>MAASGLDHLKNGYRRRFCRPSRARDINTEQGQNVLEILQDCFEEKSLANDFSTNSTKSVPNSTRKIKDTCIQSPSKECQKSHPKSVPVSSKKKEASLQFVVEPSEATNRSVQAHEVHQKILATDVSSKNTPDSKKISSRNINDHHSEADEEFYLSVGSPSVLLDAKTSVSQNVIPSSAQKRETYTFENSVNMLPSSTEVSVKTKKRLNFDDKVMLKKIEIDNKVSDEEDKTSEGQERKPSGSSQNRIRDSEYEIQRQAKKSFSTLFLETVKRKSESSPIVRHAATAPPHSCPPDDTKLIEDEFIIDESDQSFASRSWITIPRKAGSLKQRTISPAESTALLQGRKSREKHHNILPKTLANDKHSHKPHPVETSQPSDKTVLDTSYALIGETVNNYRSTKYEMYSKNAEKPSRSKRTIKQKQRRKFMAKPAEEQLDVGQSKDENIHTSHITQDEFQRNSDRNMEEHEEMGNDCVSKKQMPPVGSKKSSTRKDKEESKKKRFSSESKNKLVPEEVTSTVTKSRRISRRPSDWWVVKSEESPVYSNSSVRNELPMHHNSSRKSTKKTNQSSKNIRKKTIPLKRQKTATKGNQRVQKFLNAEGSGGIVGHDEISRCSLSEPLESDEADLAKKKNLDCSRSTRSSKNEDNIMTAQNVPLKPQTSGYTCNIPTESNLDSGEHKTSVLEESGPSRLNNNYLMSGKNDVDDEEVHGSSDDSKQSKVIPKNRIHHKLVLPSNTPNVRRTKRTRLKPLEYWRGERIDYQGRPSGGFVISGVLSPDTISSKRKAKENIGKVNKKSNKKRICLDNDERKTNLMVNLGIPLGDPLQPTRVKDPETREIILMDLVRPQDTYQFFVKHGELKVYKTLDTPFFSTGKLILGPQEEKGKQHVGQDILVFYVNFGDLLCTLHETPYILSTGDSFYVPSGNYYNIKNLRNEESVLLFTQIKR[2x];> MEEQPQMQDADEPADSGGEGRAGGPPQVAGAQAACSEDRMTLLLRLRAQTKQQLLEYKSMVDASEEKTPEQIMQEKQIEAKIEDLENEIEEVKVAFEIKKLALDRMRLSTALKKNLEKISRQSSVLMDNMKHLLELNKLIMKSQQESWDLEEKLLDIRKKRLQLKQASESKLLEIQTEKNKQKIDLDSMENSERIKIIRQNLQMEIKITTVIQHVFQNLILGSKVNWAEDPALKEIVLQLEKNVDMM;> MSPQKRVKNVQAQNRTSQGSSSFQTTLSAWKVKQDPSNSKNISKHGQNNPVGDYEHADDQAEEDALQMAVGYFEKGPIKASQNKDKTLEKHLKTVENVAWKNGLASEEIDILLNIALSGKFGNAVNTRILKCMIPATVISEDSVVKAVSWLCVGKCSGSTKVLFYRWLVAMFDFIDRKEQINLLYGFFFASLQDDALCPYVCHLLYLLTKKENVKPFRVRKLLDLQAKMGMQPHLQALLSLYKFFAPALISVSLPVRKKIYFKNSENLWKTALLAVKQRNRGPSPEPLKLMLGPANVRPLKRKWNSLSVIPVLNSSSYTKECGKKEMSLSDCLNRSGSFPLEQLQSFPQLLQNIHCLELPSQMGSVLNNSLLLHYINCVRDEPVLLRFYYWLSQTLQEECIWYKVNNYEHGKEFTNFLDTIIRAECFLQEGFYSCEAFLYKSLPLWDGLCCRSQFLQLVSWIPFSSFSEVKPLLFDHLAQLFFTSTIYFKCSVLQSLKELLQNWLLWLSMDIHMKPVTNSPLETTLGGSMNSVSKLIHYVGWLSTTAMRLESNNTFLLHFILDFYEKVCDIYINYNLPLVVLFPPGIFYSALLSLDTSILNQLCFIMHRYRKNLTAAKKNELVQKTKSEFNFSSKTYQEFNHYLTSMVGCLWTSKPFGKGIYIDPEILEKTGVAEYKNSLNVVHHPSFLSYAVSFLLQESPEERTVNVSSIRGKKWSWYLDYLFSQGLQGLKLFIRSSVHHSSIPRAEGINCNNQY;> MNQEDLDPDSTTDVGDVTNTEEELIRECEEMWKDMEECQNKLSLIGTETLTDSNAQLSLLIMQVKCLTAELSQWQKKTPETIPLTEDVLITLGKEEFQKLRQDLEMVLSTKESKNEKLKEDLEREQRWLDEQQQIMESLNVLHSELKNKVETFSESRIFNELKTKMLNIKEYKEKLLSTLGEFLEDHFPLPDRSVKKKKKNIQESSVNLITLHEMLEILINRLFDVPHDPYVKISDSFWPPYVELLLRNGIALRHPEDPTRIRLEAFHQ;> MDSYSAPESTPSASSRPEDYFIGATPLQKRLESVRKQSSFILTPPRRKIPQCSQLQEDVDPQKVAFLLHKQWTLYSLTPLYKFSYSNLKEYSRLLNAFIVAEKQKGLAVEVGEDFDIKVIFSTLLGMKGTQRDPEAFLVQIVSKSQLPSENREGKVLWTGWFCCVFGDSLLETVSEDFTCLPLFLANGAESNTAIIGTWFQKTFDCYFSPLAINAFNLSWMAAMWTACKMDHYVATTEFLWSVPCSPQSLDISFAIHPEDAKALWDSVHKTPGEVTQEEVDLFMDCLYSHFHRHFKIHLSATRLVRVSTSVASAHTDGKIKILCHKYLIGVLAYLTELAIFQIE;> MSVLRPLDKLPGLNTATILLVGTEDALLQQLADSMLKEDCASELKVHLAKSLPLPSSVNRPRIDLIVFVVNLHSKYSLQNTEESLRHVDASFFLGKVCFLATGAGRESHCSIHRHTVVKLAHTYQSPLLYCDLEVEGFRATMAQRLVRVLQICAGHVPGVSALNLLSLLRSSEGPSLEDL;> MDETVAEFIKRTILKIPMNELTTILKAWDFLSENQLQTVNFRQRKESVVQHLIHLCEEKRASISDAALLDIIYMQFHQHQKVWDVFQMSKGPGEDVDLFDMKQFKNSFKKILQRALKNVTVSFRETEENAVWIRIAWGTQYTKPNQYKPTYVVYYSQTPYAFTSSSMLRRNTPLLGQALTIASKHHQIVKMDLRSRYLDSLKAIVFKQYNQTFETHNSTTPLQERSLGLDINMDSRIIHENIVEKERVQRITQETFGDYPQPQLEFAQYKLETKFKSGLNGSILAEREEPLRCLIKFSSPHLLEALKSLAPAGIADAPLSPLLTCIPNKRMNYFKIRDK;> MEQANPLRPDGESKGGVLAHLERLETQVSRSRKQSEELQSVQAQEGALGTKIHKLRRLRDELRAVVRHRRASVKACIANVEPNQTVEINEQEALEEKLENVKAILQAYHFTGLSGKLTSRGVCVCISTAFEGNLLDSYFVDLVIQKPLRIHHHSVPVFIPLEEIAAKYLQTNIQHFLFSLCEYLNAYSGRKYQADRLQSDFAALLTGPLQRNPLCNLLSFTYKLDPGGQSFPFCARLLYKDLTATLPTDVTVTCQGVEVLSTSWEEQRASHETLFCTKPLHQVFASFTRKGEKLDMSLVS;> MDAELAEVRALQAEIAALRRACEDPPAPWEEKSRVQKSFQAIHQFNLEGWKSSKDLKNQLGHLESELSFLSTLTGINIRNHSKQTEDLTSTEMTEKSIRKVLQRHRLSGNCHMVTFQLEFQILEIQNKERLSSAVTDLNIIMEPTECSELSEFVSRAEERKDLFMFFRSLHFFVEWFEYRKRTFKHLKEKYPDAVYLSEGPSSCSMGIRSASRPGFELVIVWRIQIDEDGKVFPKLDLLTKVPQRALELDKNRAIETAPLSFRTLVGLLGIEAALESLIKSLCAEENN;> MSGKANASKKNAQQLKRNPKRKKDNEEVVLSENKVRNTVKKNKNHLKDLSSEGQTKHTNLKHGKTAASKRKTWQPLSKSTRDHLQTMMESVIMTILSNSIKEKEEIQYHLNFLKKRLLQQCETLKVPPKKMEDLTNVSSLLNMERARDKANEEGLALLQEEIDKMVETTELMTGNIQSLKNKIQILASEVEEEEERVKQMHQINSSGVLSLPELSQKTLKAPTLQKEILALIPNQNALLKDLDILHNSSQMKSMSTFIEEAYKKLDAS;> MPVKRSLKLDGLLEENSFDPSKITRKKSVITYSPTTGTCQMSLFASPTSSEEQKHRNGLSNEKRKKLNHPSLTESKESTTKDNDEFMMLLSKVEKLSEEIMEIMQNLSSIQALEGSRELENLIGISCASHFLKREMQKTKELMTKVNKQKLFEKSTGLPHKASRHLDSYEFLKAILN;> MEEEAETEEQQRFSYQQRLKAAVHYTVGCLCEEVALDKEMQFSKQTIAAISELTFRQCENFAKDLEMFARHAKRTTINTEDVKLLARRSNSLLKYITDKSEEIAQINLERKAQKKKKSEDGSKNSRQPAEAGVVESEN;> MADHNPDSDSTPRTLLRRVLDTADPRTPRRPRSARAGARRALLETASPRKLSGQTRTIARGRSHGARSVGRSAHIQASGHLEEQTPRTLLKNILLTAPESSILMPESVVKPVPAPQAVQPSRQESSCGSLELQLPELEPPTTLAPGLLAPGRRKQRLRLSVFQQGVDQGLSLSQEPQGNADASSLTRSLNLTFATPLQPQSVQRPGLARRPPARRAVDVGAFLRDLRDTSLAPPNIVLEDTQPFSQPMVGSPNVYHSLPCTPHTGAEDAEQAAGRKTQSSGPGLQKNSPGKPAQFLAGEAEEVNAFALGFLSTSSGVSGEDEVEPLHDGVEEAEKKMEEEGVSVSEMEATGAQGPSRVEEAEGHTEVTEAEGSQGTAEADGPGASSGDEDASGRAASPESASSTPESLQARRHHQFLEPAPAPGAAVLSSEPAEPLLVRHPPRPRTTGPRPRQDPHKAGLSHYVKLFSFYAKMPMERKALEMVEKCLDKYFQHLCDDLEVFAAHAGRKTVKPEDLELLMRRQGLVTDQVSLHVLVERHLPLEYRQLLIPCAYSGNSVFPAQ;> MAPRGRRRPRPHRSEGARRSKNTLERTHSMKDKAGQKCKPIDVFDFPDNSDVSSIGRLGENEKDEETYETFDPPLHSTAIYADEEEFSKHCGLSLSSTPPGKEAKRSSDTSGNEASEIESVKISAKKPGRKLRPISDDSESIEESDTRRKVKSAEKISTQRHEVIRTTASSELSEKPAESVTSKKTGPLSAQPSVEKENLAIESQSKTQKKGKISHDKRKKSRSKAIGSDTSDIVHIWCPEGMKTSDIKELNIVLPEFEKTHLEHQQRIESKVCKAAIATFYVNVKEQFIKMLKESQMLTNLKRKNAKMISDIEKKRQRMIEVQDELLRLEPQLKQLQTKYDELKERKSSLRNAAYFLSNLKQLYQDYSDVQAQEPNVKETYDSSSLPALLFKARTLLGAESHLRNINHQLEKLLDQG;> MALSTIVSQRKQI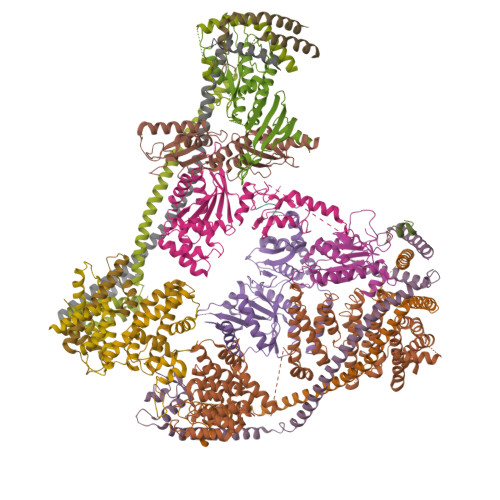KRKAPRGFLKRVFKRKKPQLRLEKSGDLLVHLNCLLFVHRLAEESRTNACASKCRVINKEHVLAAAKVILKKSRG;> MEGAGAGSGFRKELVSRLLHLHFKDDKTKVSGDALQLMVELLKVFVVEAAVRGVRQAQAEDALRVDVDQLEKVLPQLLLDF adenosine 5'-heptaphosphate | C10 H20 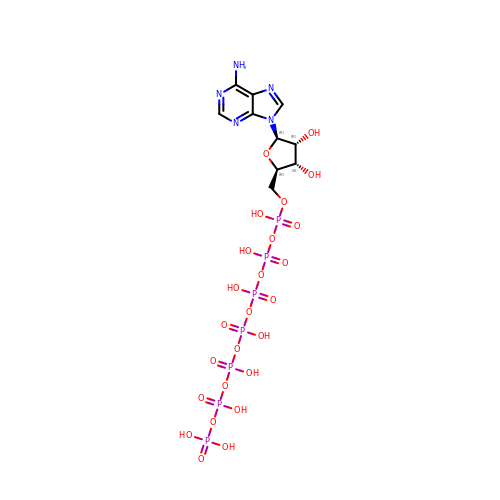N5 O25 P7 | CLTPWCJSZCAWDP-KQYNXXCUSA-N> GSAMGNYMGNPWTEYMAKYDIEEVHGSGIRVDLGEDAEVAGTQYRLPSGKCPVFGKGIIIENSNTTFLTPVATGNQYLKDGGFAFPPTEPLMSPMTLDEMRHFYKDNKYVKNLDELTLCSRHAGNMIPDNDKNSNYKYPAVYDDKDKKCHILYIAAQENNGPRYCNKDESKRNSMFCFRPAKDISFQNYTYLSKNVVDNWEKVCPRKNLQNAKFGLWVDGNCEDIPHVNEFPAIDLFECNKLVFELSASDQPKQYEQHLTDYEKIKEGFKNKNASMIKSAFLPTGAFKADRYKSHGKGYNWGNYNTETQKCEIFNVKPTCLINNSSYIATTALSHPIEVEAAALVPR;> DITQQAKDIGAGPVASCFTTRMSPPQQICLNSVVNTALS

The formation of a moving junction (MJ) between the membranes of the parasite and its host cell is essential for invasion. Two important components of the MJ are Apical Membrane Antigen 1 (AMA1) on the parasite surface and the Plasmodium rhoptry neck (RON) protein complex that is translocated to the erythrocyte membrane during invasion. The extra-cellular region of RON2, a component of this complex, interacts with AMA1, providing a bridge between the parasite and its host cell that is crucial for successful invasion. Here, we report the crystal structure of the complex formed between PfAMA1 and peptide segments of PfRON2, which, together with our previous structural results on the TgAMA1-TgRON2 co-structure, highlights a conserved, crucial interaction in apicomplexan host cell invasion.

From the 67-residue construct, PfRON2-5, that we previously showed to have affinity for PfAMA1, and guided by the TgAMA1-TgRON2sp structure, we synthesized two analogous PfRON2 peptides: PfRON2sp1 (residues 2021–2059; numbering from the initiation methionine in PF14_0495), and PfRON2sp2 (residues 2027–2055). PfRON2sp1 and PfRON2sp2 were co-crystallized with the first two ectoplasmic domains (DI, DII) of recombinant PfAMA1 3D7 or CAMP strains, respectively. PfRON2sp1, traced from Thr2023 to Leu2058, includes a disulfide bridge between Cys2037 and Cys2049 and makes several direct contacts with PfAMA1, resulting in a total buried surface area of 3154 Å2 (1441 Å2 for PfAMA1 and 1713 Å2 for PfRON2sp1). Overall, the binding paradigm established by TgAMA1-TgRON2sp is maintained, with an N-terminal helix seated at one end of the AMA1 receptor-binding groove and extended through an ordered coil to a disulfide-closed β-hairpin loop, generating a U-shaped conformation. Similarly, exposing a functional receptor-binding groove on AMA1 requires displacement of the extended non-polymorphic DII loop, which adopts a disordered state (not modeled between Lys351 to Ala387); this region is stabilized by DI in apo PfAMA1. Intriguingly, the backbone of the N-terminal helix and additional coil of PfRON2sp1 (2024-QQAKDIGAG-2032) overlays remarkably well with a section of the apo PfAMA1 DII loop (360-YEKIKEGFK-368) (rmsd<0.4 Å), which also includes a helical region. The majority of intermolecular contacts are formed by the segment Lys2027-Met2042 of PfRON2sp1. An influential residue on PfRON2 appears to be Arg2041, a residue specific to the P. falciparum species, located at the tip of the β-hairpin with its guanidyl group fitting snugly into a preformed pocket of PfAMA1. An additional feature of the PfRON2sp cystine loop region is the presence of a cis peptide bond between Ser2043 and Pro2044; the Ser-Pro-Pro segment contributes negligible buried surface area but is important for maintaining the β-hairpin conformation for efficient complex formation. Since PfRON2sp1 is more biologically relevant than its truncated counterpart, it is used for the following analyses unless otherwise noted.>[2x]MYKEPFGVKVDFETGIIEGAKKSVRRLSDMEGYFVDERAWKELVEKEDPVVYEVYAVEQEEKEGDLNFATTVLYPGKVGKEFFFT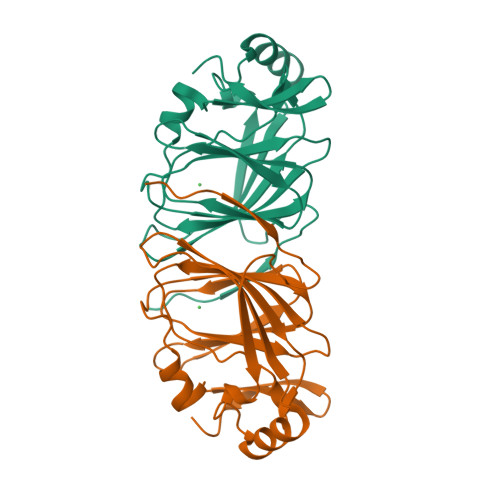KGHFHAKLDRAEVYVALKGKGGMLLQTPEGDAKWISMEPGTVVYVPPYWAHRTVNIGDEPFIFLAIYPADAGHDYGTIAEKGFSKIVIEENGEVKVVDNPRWKK> MLKLAIPKGRLEEKVMTYLKKTGVIFERESSILREGKDIVCFMVRPFDVPTYLVHGVADIG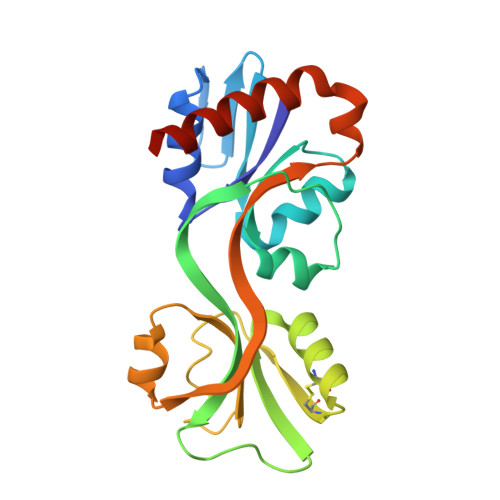FCGTDVLLEKETSLIQPFFIPTNISRMVLAGPKGRGIPEGEKRIATKFPNVTQRYCESKGWHCRIIPLKGSVELAPIAGLSDLIVDITETGRTLKENNLEILDEIFVIRTHVVVNPVSYRTKREKVVSFLEKLQEVIEHDSNEQSRG>[4x]MQSLAKL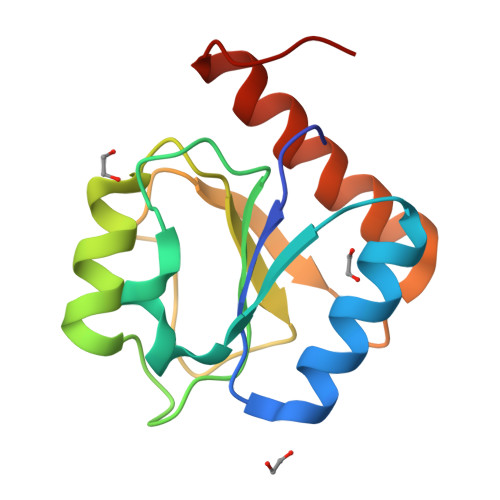LVIEDDAAIRLNLSVILEFVGEQCEVIESTQIDQINWSAVWGGCILGSLRGQALSEQLIQSLTKANHIPLLVANKQPYSLEEFPNYVGELDFPLNYPQLSDALRHCKEFLGRKGFQVLAT>GPKFPRVKNWELGSITYDTLCAQSQQDGPCTPRRCLGSLVLPRKLQTRPSPGPPPAEQLLSQARDFINQYYSSIKRSGSQAHEERLQEVEAEVASTGTYHLRESELVFGAKQAWRNAPRCVGRIQWGKLQVFDARDCSSAQEMFTYICNHIKYATNRGNLRSAITVFPQRAPGRGDFRIWNSQLVRYAGYRQQDGSVRGDPANVEITELCIQHGWTPGNGRFDVLPLLLQAPDEAPELFVLPPELVLEVPLEHPTLEWFAALGLRWYALPAVSNMLLEIGGLEFSAAPFSGWYMSTEIGTRNLCDPHRYNILEDVAVCMDLDTRTTSSLWKDKAAVEINLAVLHSFQLAKVTIVDHHAATVSFMKHLDNEQKARGGCPADWAWIVPP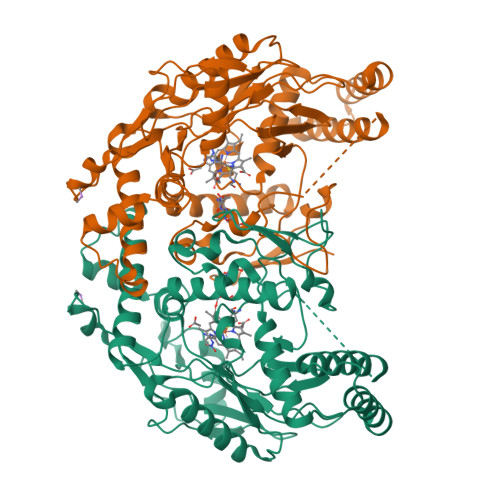ISGSLTPVFHQEMVNYILSPAFRYQPDPWK[2x]> MASSLQSKWICLRLNDAIIKRHVLVLSEYADLKYLGFEKYKFFEYVIFQFCNDPQLCKIIENNYNYCMQIFKAPADDMRDIRHNIKRAFKTPVLGHMCVLSNKPPMYSFLKEWFLLPHYKVVSLKSESLTWGFPHVVVFDLDSTLITEEEQVEIRDPFVYDSLQELHEMGCVLVLWSYGSRDHVAHSMRDVDLEGYFDIIIS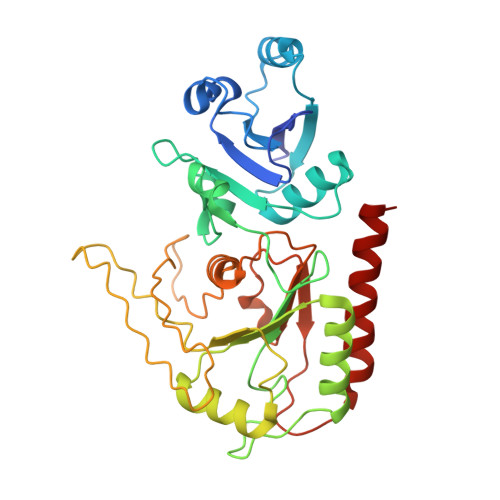EGSTVQEERSDLVQNSHNAIVDYNLKKRFIENKFVFDIHNHRSDNNIPKSPKIVIKYLSDKNVNFFKSITLVDDLPTNNYAYDFYVKVKRCPTPVQDWEHYHNEIIQNIMDYEQYFIK>[4x]MSSATPDPAEILTARKAVGLSQTAAAALVHSSLRTWQQWEAGDRRMHPGLWELFLLKTQLPSPSS

Many acr genes form an operon with genes encoding transcriptional regulators, called anti-CRISPR-associated (Aca) proteins. Aca10 is the most recently identified Aca family that is suggested as a transcriptional regulator by controlling the expression of acrIC7 and acrIC6 in P. citronellolis and in other analogous contexts. In conclusion, Aca10 from P. citronellolis is a dimeric DNA binding protein and a likely transcriptional repressor of the acrIC7-acrIC6-aca10 operon. Aca10 forms a dimer in solution and the dimeric form is critical for binding specific DNA.

The diffraction data were collected at a resolution of 1.76 Å at PAL synchrotron. The crystal belonged to space group P41212 and four molecules were present in the asymmetric unit (ASU). The final structural model contained most of the Aca10 sequence (residues from S3 to L60 out of 65 amino acids) for all four molecules. The structure of Aca10 showed that it was constructed of an α-helical bundle fold comprising four α-helices (α1−α4). Analysis of the surface electrostatic potential of Aca10 showed that most was positively charged, whereas one face composed of α4 and a connected loop was highly negatively charged. The AB dimer was a symmetric dimer, whereas the BC dimer was asymmetric. Since DNA-binding proteins, especially those recognizing palindromic DNA sequences, are typically symmetric dimers, the AB dimer was the more likely biologically relevant form. The PPI, mainly constructed by helix α4 from both molecules, was formed by multiple hydrogen bonds and salt bridges. Salt bridges formed by residues H30, E52 and K57 from each molecule were the primary forces maintaining the integrity of this dimeric interface. R44 in the connected loop between α3 helix and α4 helix is a critical residue involved in the DNA binding, which likely results in a high degree of DNA bending.The C-type mannose receptor and its homolog Endo180 (or uPARAP, for urokinase plasminogen activator receptor-associated protein) mediate the endocytic uptake of collagen by macrophages and fibroblasts. The large extracellular region of each of these receptors consists of an N-terminal ricin B-like domain, followed by a fibronectin type II (FN2) domain and eight (MR, Endo180, PLA2R) or ten (DEC-205) C-type lectin (CTL) domains. Here, we present the crystal and solution structures of domains 1–4 (D1-4) of Endo180 and a mutational analysis of collagen binding. The Endo180 D1-4 region adopts an L-shaped structure with a short arm (∼60 Å length) consisting of the ricin-like and FN2 domains, and a longer arm (∼80 Å length) consisting of the two CTL domains.

We obtained two crystal forms of the natively glycosylated D1-4 region, one of which diffracted to 2.5 Å resolution and allowed the structure to be determined. The overall structure of Endo180 D1-4 is the same in both crystal forms (the root-mean-square deviations [rmsd] between the four crystallographically independent copies range from 1.2 to 1.4 Å) and only the high-resolution structure is described in the following. We have determined the crystal structure at 2.5 Å resolution of the N-terminal region of Endo180, consisting of a ricin-like domain, a fibronectin type II (FN2) domain, and two C-type lectin (CTL) domains. The L-shaped arrangement of these domains creates a shallow trench spanning the FN2 and CTL1 domains, which was shown by mutagenesis to bind triple-helical and denatured collagen. The inter-domain interfaces are sizable (ricin-FN2, 552 Å2; FN2-CTL1, 674 Å2; CTL1-CTL2, 662 Å2), suggestive of a stable arrangement with limited inter-domain flexibility. There is no electron density for residues 101–104 and 137–155 in the ricin-like domain and residues 364–378 in the CTL1-CTL2 linker. The D1-4 region contains five predicted N-linked glycosylation sites. We observed weak electron density for the glycans at Asn69 and Asn497; the glycosylation sites at Asn102, Asn140, and Asn364 are located in the disordered loop regions mentioned above. No Ca2+ ions were present in our crystallization solution, but we observed electron density for a metal ion (most likely Na+) in each CTL domain in a position corresponding to the canonical Ca2+ “site 2” (Weis et al., 1998). The Na+ ions in Endo180 are coordinated by Gln326, Asp328, Glu333, and Asn348 in CTL1, and by Glu470, Asn472 and Asp493 in CTL2. Comparison with a typical Ca2+-loaded CTL domain structure suggests that the Endo180 D1-4 crystal structure is unlikely to change much upon Ca2+ binding.

>[2x]APLADAALPEPNVFLIFSHGLQGCLEAQGGQVRVTPACNTSLPAQRWKWVSRNRLFNLGTMQCLGTGWPGTNTTASLGMYECDREALNLRWHCRTLGDQLSLLLGARTSNISKPGTLERGDQTRSGQWRIYGSEEDLCALPYHEVYTIQGNSHGKPCTIPFKYDNQWFHGCTSTGREDGHLWCATTQDYGKDERWGFCPIKSNDCETFWDKDQLTDSCYQFNFQSTLSWREAWASCEQQGADLLSITEIHEQTYINGLLTGYSSTLWIGLNDLDTSGGWQWSDNSPLKYLNWESDQPDNPSEENCGVIRTESSGGWQNRDCSIALPYVCKKKPNATAEPTPPDRWANVKVECEPSWQPFQGHCYRLQAEKRSWQESKKACLRGGGDLVSIHSMAELEFITKQIKQEVEELWIGLNDLKLQMNFEWSDGSLVSFTHWHPFEPNNFRDSLEDCVTIWGPEGRWNDSPCNQSLPSICKKAGQLSG> MSGQQHSSDNKNWAEKGIVIREVEILGKRPMKDIGVQQTRFDSLVLKENIALSMADILTFNSSIFVKSYGRATLSTVSFRGTSASHTQVTWNGMRINNPMLGMTDFSMIPSYFIDDASLLHGTSSVNMAGGGLGGLVKLSTVPAHQEGFGMQYVQGIGSFSTFDEFLQLKYGDKHWQISTRAVYQSSPNDYKYRNHDKKENIYDDKYNIIEQYYPIERNRSGAYKDLHILQEVYYNTGKGDRFGLNAWYTDSNRELALLTTDQGDLMDFENRQREHTLRSVLSWDHTRENWKVSARGGYVHTWLAYDYKRDLGNGIMATMTRSRSKVNTFYGQLDGEYFFSDKLLLTAGVSAHQHLVNSLDKDLNKDDNKNDKYGQGRKNDSIVYFDKGRIELSGNVSLKWQPVNRLGMSLVLRGEMFGTKWAPVIPAFFVDYVLSKRGNIM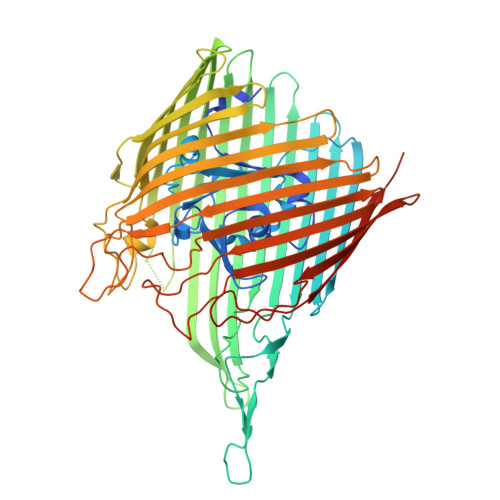AKASITRNYRFPTLNDLYFLPGGNPALNNESGFTYETGLSFSVDKDNVYTLSGSASWFDQHINDWIIWLPTSKGFYSPVNLKKVHAYGVEVQADYAVAIDKAWKLGLNGTFAWTPSINEGEPTSKADQSVGKQLPYIPEYSATLSGRLTYRSWGLLYKWCYYSERYTMTSNAVSYTGHLPPYLMSNVTLEKGFSLRWADLSLKGTVNNLFDEEYLSVLSRPMPGINFEFFIGITPKWGKKKKGGGHHHHHH> HSSGLVPRGSHMAIIFPGQGAQKVGMAQDLFNNNDQATEILTSAAKTLDFDILETMFTDEEGKLGETENT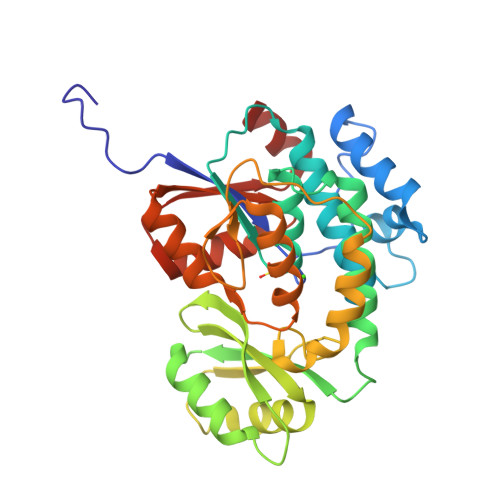QPALLTHSSALLAALKNLNPDFTMGHSLGEYSSLVAADVLSFEDAVKIVRKRGQLMAQAFPTGVGSMAAVLGLDFDKVDEICKSLSSDDKIIEPANINCPGQIVVSGHKALIDELVEKGKSLGAKRVMPLAVSGPFHSSLMKVIEEDFSSYINQFEWRDAKFPVVQNVNAQGETDKEVIKSNMVKQLYSPVQFINSTEWLIDQGVDHFIEIGPGKVLSGLIKKINRDVKLTSIQTLEDVKGWNEND>MATTSNQNVEFVRTGYGKNMVKVLHIRREGNHHHIIELIANVQLTLKTRKDYLTGDNSDIIPTDTVKNTVHALAKLKGIKSIESFALDICEHFLTAFNHVTRVKVNIDEVPWKRLEKNGVEHNHAFIHCPEALRFCEAEQYLSKTPVVHSGLKDMKVLKTTQTGFEGFLRDRFTTLTDAKDRFFCTSVYARWRYNTINVAFDAAWKAVKDTVIQKFAGPYDRGEYSPSVQKTLYDTQLLVLDRIPEVEEIEIIMPNQHYFVIDMTKIGLSNKDEVYLPLDNPSGNITGTVCRKPRARM[8x]

Urate oxidase (uricase, Uox) catalyses hydroxylation of urate to give 5-hydroxyisourate (HIU). This is the first and rate-limiting step of uricolysis, a three-step enzymatic pathway present in both prokaryotes and eukaryotes that converts urate into the more soluble (S)-allantoin. The oldest known structure of the enzyme is a tetramer of the tunnelling (T) fold domain able to catalyse urate oxidation without the help of cofactors. The zebrafish (Danio rerio) urate oxidase (chr11: 8151055.8158017) encodes a protein of 298 aa with a C-terminal tripetide (ARM) corresponding to the type 1 peroxisome-targeting signal.

The crystal structure of DrUox was obtained at 2.8 Å resolution with a continuous electron density from Gly8 to Pro294. The DrUox structure shows the typical T-fold with a homotetramer organized as a dimer of dimers joining head-to-head to form the functional tetramer. Each monomer contains two tandem repeats of the T-fold domain forming an antiparallel β8-sheet with four main α-helices located at the concave side of the sheet. Two monomers assemble into a dimer by a two-fold axis to form a β16α8 barrel. The main dimerization interface is an antiparallel β-sheet formed by the N-terminal (aa 8–20) and C-terminal (aa 282–293) β strands of two subunits. The active sites (four in the tetramer) are located at the dimerization interfaces. In the crystal structure, chains A-C and B-D at the tetramer interface are connected by a disulfide bond involving Cys129, a residue not conserved in Uox sequences. The geometrical parameters of the disulfide, classify it as having a Left-Handed Staple conformation (+LHStaple), a rare bond characterized by a high strain energy. Phenylalanine 216, a residue strictly conserved in Uox alignment, is not part of the tetramer interface, but establishes main chain and side chain interaction with lysine 158 of the tetramer interface. F216 is not directly involved in substrate binding, but is involved in a cluster of hydrophobic interactions with active site residues.>AMSKKEININNYNDDAIQVLEGLDAVRKRPGMYIGSTDGAGLHHLVWEIVDNAVDEALSGFGDRIDVTINKDGSLTVQDHGRGMPTGMHAMGIPTVEVIFTILHAGGKFGQGGYKTSGGLHGVGSSVVNALSSWLEVEITRDGAVYKQRFENGGKPVTTLKKIGTAPKSKTGTKVTFMPDATIFSTTDFKYNTISERLNESAFLLKNVTLSLTDKRTDEAIEFHYENGVQDFVSYLNEDKEILTPVLYFEGEDNGFQVEVALQYNDGFSDNILSFVNNVRTKDGGTHETGLKSAITKVMNDYARKTGLLKEKDKNLEGSDYREGLAAVLSILVPEEHLQFEGQTKDKLGSPLARPVVDGIVADKLTFFLMENGELASNLIRKAIKARDAREAARKARDESRNGHHHHHH[2x]

Bacteria usually express two highly conserved type IIA topoisomerases (Top2As), topoisomerase (topo) IV and DNA gyrase, involved respectively in chromosome relaxation/segregation and DNA supercoiling. Topo IV is a tetramer composed of two subunits, ParC and ParE, that form an active E2C2 complex; likewise gyrase through GyrA and GyrB subunits. Topo2As introduce a transient 4 bp staggered break into one DNA duplex and pass a second DNA duplex through the break which is then resealed. In this study, we have co-crystallized the ParE ATPase domain with short DNA duplexes in the presence of adenosine 5'-[β,γ-imido]triphosphate Adenylyl-imidodiphosphate (AMP-PNP), a non-hydrolysable ATP analogue that induces dimerization of ATPase domains to close the ATPase gate.

Comparison of the ParE hole in the 14-mer hole-bound and 6-mer outside-bound structures showed that hole binding by DNA did not significantly alter the dimensions of the cavity and that the side-bound DNAs interact weakly with adjacent dimers in the crystal lattice. By comparison, for the side-bound DNA-ParE44 complex, the B factors on DNA and protein are 69 Å2 and 27 Å2, indicating tighter binding of the side-bound DNA, possibly enhanced by DNA interactions between adjacent dimers in the crystal. However, importantly we note that the side binding of DNA to ParE occurs exclusively through K291, R321, and K346 and K281, i.e., an exact subset of the residues seen in the hole-bound DNA complex and shown by mutagenesis of 291, 321 and 346 to be important for enzyme activity. The biological role of side-bound DNA is not immediately clear. We propose that binding first occurs through the side-bound DNA process and is crucial for initial stabilization of the T segment (reflected in the higher impact of mutation of the protein residues involved). Another new finding is that certain short DNA duplexes, including the hole-binding 14-mer, are sufficient to stimulate the topo IV ATPase activity whereas other duplexes, e.g., 5′-GCGCGC, were inactive.>ATAQQASGVRATYNYYNPTQNNWDLAGTYCATWDAGQPLSWRSKYGWTAFCGPAGPTGQAACGQCLLVTNTATGA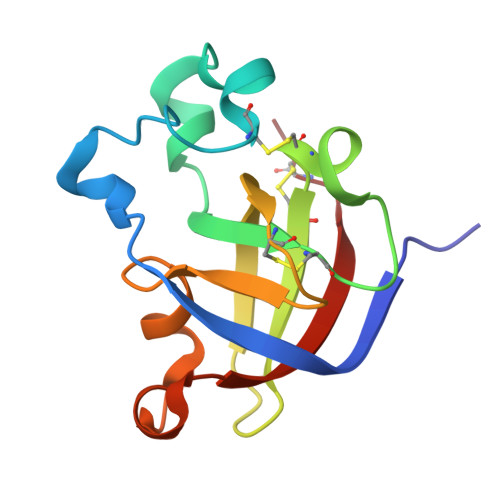SLTVRIVDQCSNGGLDLDYDTAFKPLDTNGAGIQAGHLTVNYQFVNCGN[2x]(2Z,6Z,10Z,14Z,18Z,22Z,26Z)-3,7,11,15,19,23,27,31-octamethyldotriaconta-2,6,10,14,18,22,26,30-octaen-1-yl trihydrogen diphosphate | C40 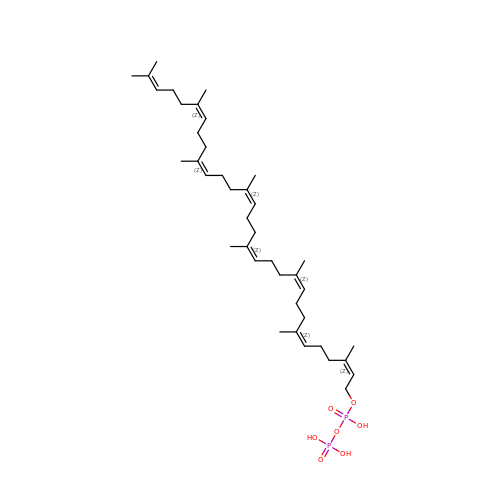H68 O7 P2 | IKKLDISSULFFQO-DLTKSLTJSA-N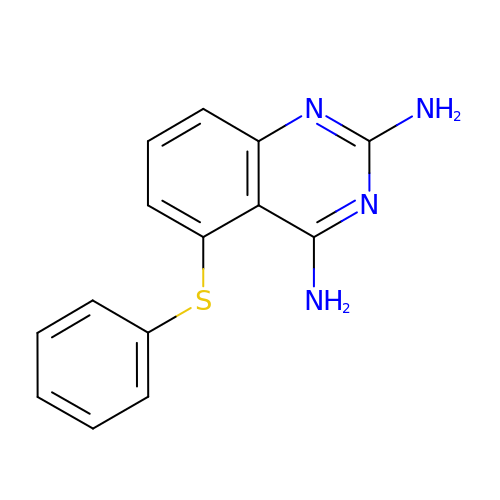5-PHENYLSULFANYL-2,4-QUINAZOLINEDIAMINE | C14 H12 N4 S | BUFDQCGCADQQQY-UHFFFAOYSA-N> GPLGSMFHVRYRMEASCLELALEGERLCKSGDCRAGVSFFEAAVQV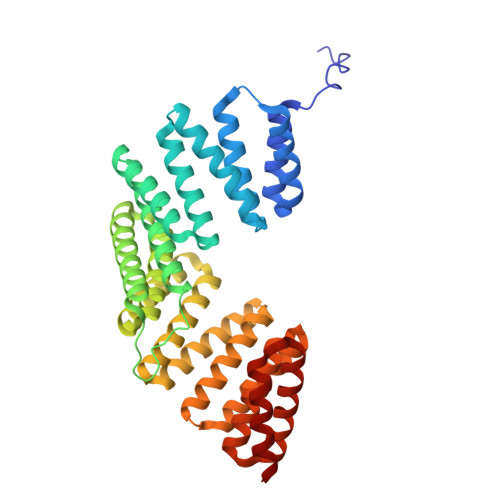GTEDLKTLSAIYSQLGNAYFYLHDYAKALEYHHHDLTLARTIGDQLGEAKASGNLGNTLKVLGNFDEAIVCCQRHLDISRELNDKVGEARALYNLGNVYHAKGKSFGCPGPQDVGEFPEEVRDALQAAVDFYEENLSLVTALGDRAAQGRAFGNLGNTHYLLGNFRDAVIAHEQRLLIAKEFGDKAAERRAYSNLGNAYIFLGEFETASEYYKKTLLLARQLKDRAVEAQSCYSLGNTYTLLQDYEKAIDYHLKHLAIAQELNDRIGEGRACWSLGNAYTALGNHDQAMHFAEKHLEISREVGDKSGELTARLNLSDLQMV>[4x]TTVNETTPIAPAKVLPDAQTVTSVRHWTDTLFSFRVTRPQTLRFRSGEFVMIGLLDDNGKPIMRAYSIASPAWDEELEFYSIKVPDGPLTSRLQHIKVGEQIILRPKPVGTLVIDALLPGKRLWFLATGTGIAPFASLMREPEAYEKFDEVIMMHACRTVAELEYGRQLVEALQEDPLIGELVEGKLKYYPTTTREEFHHMGRITDNLASGKVFEDLGIAPMNPETDRAMVCGSLAFNVDVMKVLESY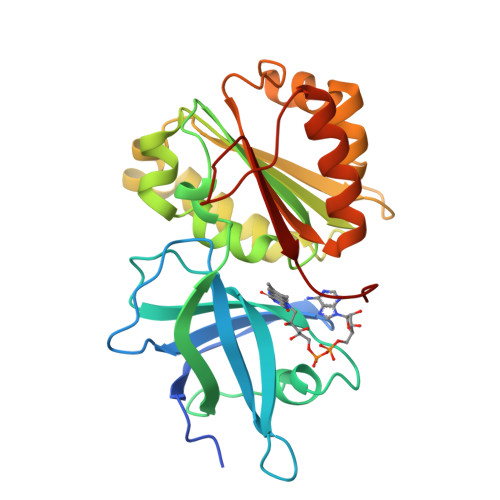GLREGANSEPREFVVEKAFVGEGI> MKLDIKKTFSNRSDRVKGIDFHPTEPWVLTTLYSGRVELWNYETQVEVRSIQVTETPVRAGKFIARKNWIIVGSDDFRIRVFNYNTGEKVVDFEAHPDYIRSIAVHPTKPYVLSGSDDLTVKLWNWENNWALEQTFEGHEHFVMCVAFNPKDPS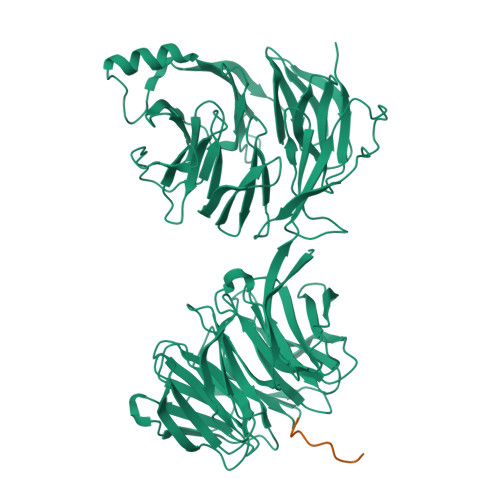TFASGCLDRTVKVWSLGQSTPNFTLTTGQERGVNYVDYYPLPDKPYMITASDDLTIKIWDYQTKSCVATLEGHMSNVSFAVFHPTLPIIISGSEDGTLKIWNSSTYKVEKTLNVGLERSWCIATHPTGRKNYIASGFDNGFTVLSLGNDEPTLSLDPVGKLVWSGGKNAAASDIFTAVIRGNEEVEQDEPLSLQTKELGSVDVFPQSLAHSPNGRFVTVVGDGEYVIYTALAWRNKAFGKCQDFVWGPDSNSYALIDETGQIKYYKNFKEVTSWSVPMHSAIDRLFSGALLGVKSDGFVYFFDWDNGTLVRRIDVNAKDVIWSDNGELVMIVNTNSNGDEASGYTLLFNKDAYLEAANNGNIDDSEGVDEAFDVLYELSESITSGKWVGDVFIFTTATNRLNYFVGGKTYNLAHYTKEMYLLGYLARDNKVYLADREVHVYGYEISLEVL;> CTFKTKTN> ENLYFQGMTFEHIISSKRLEGFLRHLAEEGVGGVEPLAKGTTSLVFTGVLGGRKVVIKLQRPDSPRSNFEKEAELTKIASTFGVTPPIIGLGEFEGLPYLIREFAEGEPILFADVEKEHLFRIVEKTALLDRLGIDHGQIQGGKHIIIGEDVYLIDFEKAGFRKPNNLTSAMAMIFIGENAISKRVREKFGL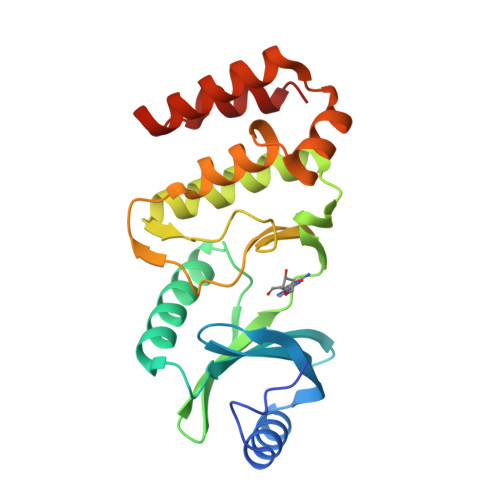DEKFREEMKDALRHYKRTGSLSRLLSLLSGL> HHHHHHSSGLVPRGSHMTDIRSET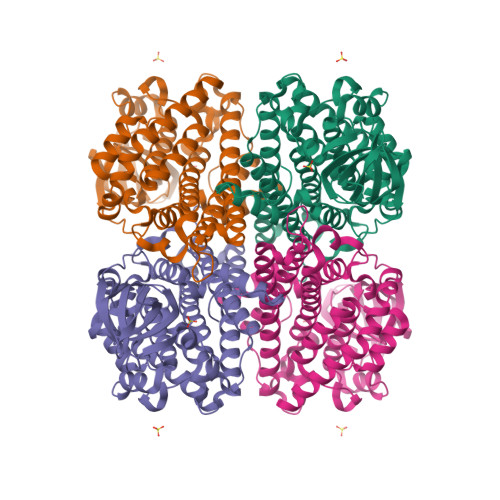AELRAELVERVHKFGPVFADGVAEGERERRLPDATVRAIDQSQLAMLWTAKSYGGLETDVRTMSEVAKVLSHYCPSTSWVVNNVNGSNLLASKFPRAALDEVFGDAPGAKLASVFAAAGTAVRTPGGYRLTGSWPYGTGILHDDWAILVAREVDADGEPVGGLSMLVPARDLTVEDTWHTVGMRATGSHTVVLRDTFVPEHRVISGELQRSRESATDLGLPPLFRTAAIAAMAVVCASVVLGAGQAARALVVEKAPTRGIAPSKYTRQTDSRTFVSSLGRTALSIDAAEMHVARAATALDDAAYDAVALPDSELLRIRGDVGQAVSLVTTALDELLWAHGAASFAESNPLQRYWRDANTAARHAMLNVHVGHELYGGSFFGLDPIVPSL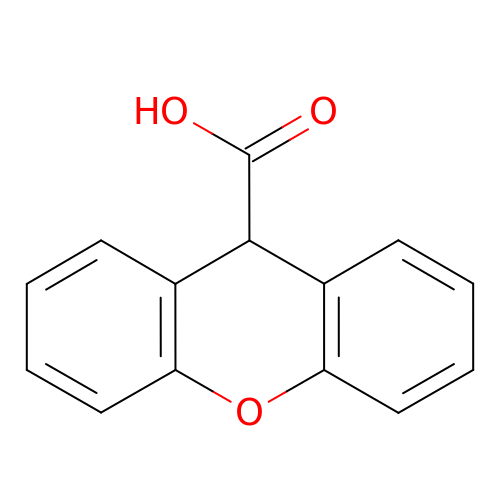9~{H}-xanthene-9-carboxylic acid | C14 H10 O3 | VSBFNCXKYIEYIS-UHFFFAOYSA-N We discover FucOB from the mucin-degrading bacteria Akkermansia muciniphila as an α-1,2-fucosidase able to hydrolyze Type I, Type II, Type III and Type V H antigens to obtain the afucosylated Bombay phenotype in vitro. FucOB displays α-1,2-L-fucosidase activity and showed no activity against α-1,3, α-1,4, and α-1,6 fucosylated oligosaccharides. A close inspection of the crystal structure revealed that FucOB crystallized as a monomer comprising three domains from the N- to the C-terminus: (i) a β-sandwich domain (residues 25–260), (ii) an (α/α)6 helical barrel catalytic domain (residues 357–712) and (iii) a second β-sandwich domain (residues 713–785). FucOB as well as other members of the GH95 family follow a single displacement inverting catalytic mechanism.

The high quality of the electron density maps allowed the trace of residues 25–785. The (α/α)6 helical barrel of FucOB displays a deep groove where the active site is located, mainly flanked by solvent-exposed and flexible loops, including loop 25 (α7−α8; residues 357–386), loop 28 (α9−α10; residues 429–458), loop 33 (β19–α13; residues 547–550), loop 35 (α14−α15; residues 587–614); loop 37 (α16−α17; residues 651-655), loop 39 (α18−α19; residues 683–699) and α-helix 8 (residues 387–392). A first glycerol molecule is deeply buried into a pocket defined by W378, H383, W655, and H693. The O1 and O2 atoms make hydrogen bonds with the side chains of N387 and Q697, respectively. A second glycerol molecule accommodates into an adjacent solvent exposed pocket mainly defined by Y106 and W453. The O3 and O2 atoms make hydrogen bonds with the side chains of S444 and H383, respectively. A third glycerol molecule is located near the first glycerol molecule. The O1, O2, and O3 atoms interact with the side chains of H693, R612, and H613, respectively. The crystal packing analysis of FucOB and FucOBE541A structures reveals a strong π–π stacking interaction between W453 with two prolines residues, P765 and P783, of the neighbor protomer. Consequently, this protomer restricts the entrance of the substrate into the active site, supporting the inability to obtain a complex crystal form.

> KPSASNLIWSDEPAVVVYPQEDKNSEGSFGKYRKPASVWEAEGYPIGNGRVGAMIFSAPGRERLALNEISLWSGGANPGGGYGYGPDAGTNQFGNYLPFGDLFVDFKKGDQPASLSVEDFTRSLDLRDGIHKVNYKADGVTYDREAFSSTPANVLVLNYKASKPGQFSADFSVNSQLGADISAKGSVITWKGMLKNGMNYEGRVLIRPKGGTLSASGDKISVKNADSCMVVIAMETDYLMDYKKDWKGESPSRKLDRYAAKAASADYAALKQAHISQYKSMFDRVKVNFGKTEEDVAKLPTPKRLEAYKKNPADPDLEETMFQFGRYLLLSSSRPGTLPANLQGLWNDYVKPPWACDYHNNINVQMAYWGAEPANLSECHEALVNYVEAMAPGCRDASQANKGFNTKDGKPVRGWTVRTSQNIFGGNGWQWNIPGAAWYALHIWEHYAFTGDRKYLEKQAYPLMKEICHFWEDHLKELGAGGEGFKTNGKDPSEEEKKDLADVKAGTLVAPNGWSPEHGPREDGVMHDQQLIAELFSNTIKAARILGKDAAWAKSLEGKLKRLAGNKIGKEGNLQEWMIDRIPKTDHRHTSHLFAVFPGNQISKLKTPKLAEAARLSLEWRGTTGDSRRSWTWPWRTALWARLGEGNKAHEMVQGLLKFNTLPNMLTTHPPMQMDGNFGIVGGICEMLVQSHAGGLDIMPSPVEAWPEGSVKGLKARGNVTVDFSWKDGKVSNVKLYSAQPKVLPVRVNGKMTRMKTLPLK> DDILSSIWTEGLLMCLIVSALL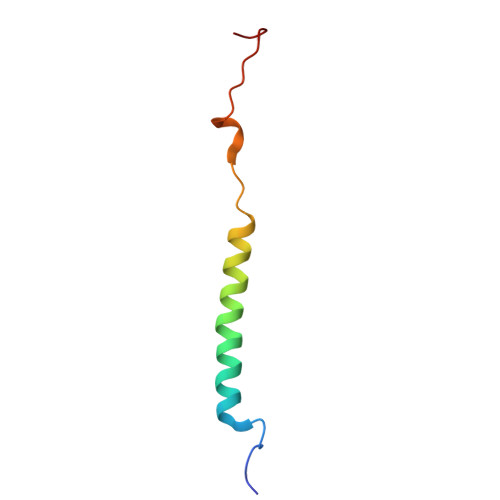LFILIVALSWISNLDITYGALEKSTNPIKK>[2x]AMAKDSKAPVVEIFDERDGCTSAGSTGKASDAGEKGLLVKVSMQKVGYNAIMAKSVAASYMNA;>[2x]LDAFSKVI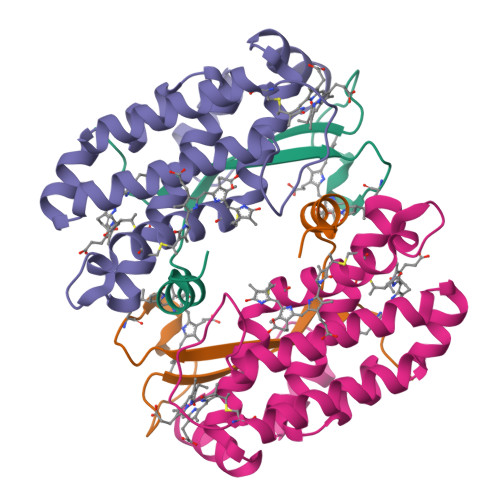TSADGKAAYVGGADLQALKKFVSDGNKRMDAVNAIVSNASCIVSDAVSGMVCENPSLIAPNGGVYSNRKMAACLRDAEIILRYVSYSLLSGDSSVLEDRCLNGLKETYSSLGVPAAGNARAVAIMKATVNSFINNTAQQKKLSVPSGDCSALASEAGGYFDKVTSAIA>[4x]MDSIGDRMKRYENAYRIKLPERMPVIVRIDGAHFHTYTKGCAKPFDQDLAEAFWETCKYLAQNIMGAKLVYHQSDEIS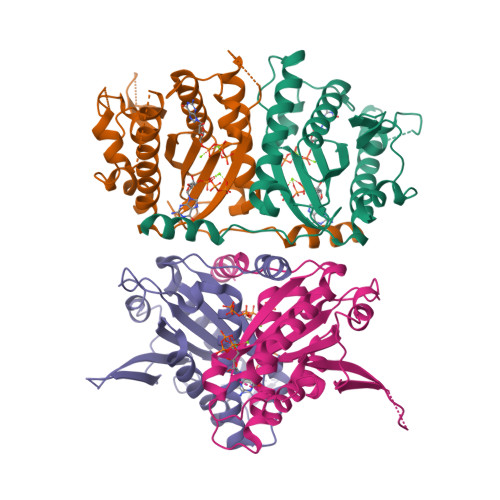ILITNYDKLTTQSWFENNLQKIASVSASMATAKFNEVMREKYPDKPLATFDGRAQVLPQDEVANYFIWRQQDASKNSISMVAQANFPHKQLQGLNGKDMQDKLMTEKNINWNDLPVWQKRGICIIKEFYEKNGALRSRWSVDHETPIISKDREYVEQFVYLNRGAAA> MKYSLCTISFRHQLISFTDIVQFAYENGFEGIELWGTHAQNLYMQEYETTERELNCLKDKTLEITMISDYLDISLSADFEKTIEKCEQLAILANWFKTNKIRTFAGQKGSADFSQQERQEYVNRIRMICELFAQHNMYVLLETHPNTLTDTLPSTLELLGEVDHPNLKINLDFLHIWESGADPVDSFQQLRPWIQHYHFKNISSADYLHVFEPNNVYAAAGNRTGMVPLFEGIVNYDEIIQEVRDTDHFA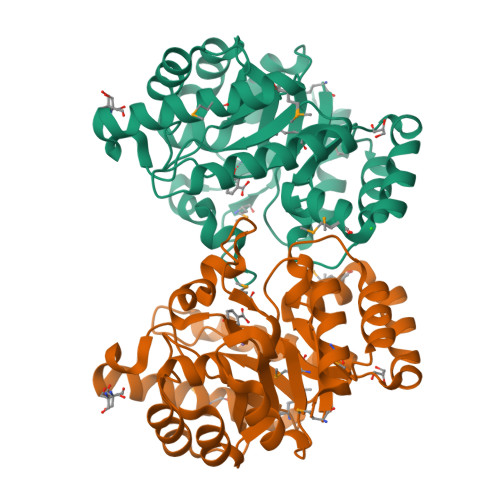SLEWFGHNAKDILKAEMKVLTNRNLEVVTSENLYFQ> GMEKLNFGIPEWAFEFHGHKCPYMPMGYRAGSYALKIAGLEKEKDHRTYLLSEMSPEDMNGCFNDGAQAATGCTYGKGLFSLLGYGKLALILYRPGRKAIRVHVRN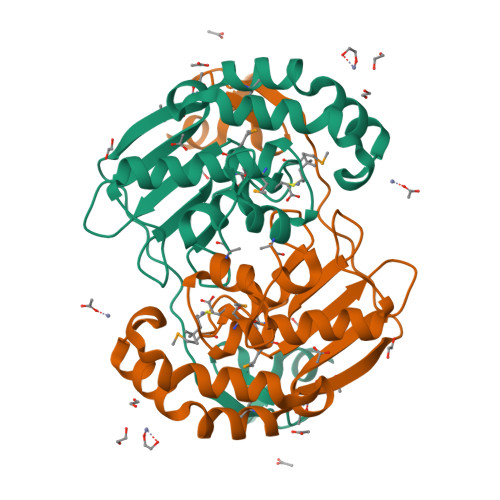SFMDELSTRASDFFRYRKQGYEPSEIPAGAIDPVLEWISSLEDEEIFEYREIDGFTFEPVKKNGAKVRCDVCGEYTYEADAKLLNGKPVCKPDYYGKK> GAMGSMSKSLKKLVEESREKNQPEVDMSDRGISNMLDVNGLFTLSHITQLVLSHNKLTMVPPNIAELKNLEVLNFFNNQIEELPTQISSLQKLKHLNLGMNRLNTLPRGFGSLPALEVLDLTYNNLSENSLPGNFFYLTTLRALYLSDNDFEILPPDIGKLTKLQIL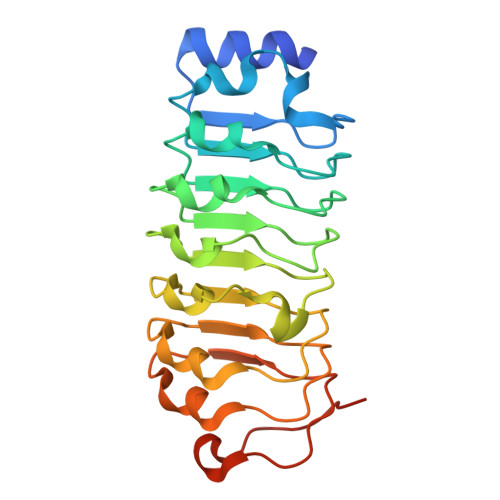SLRDNDLISLPKEIGELTQLKELHIQGNRLTVLPPELGNLDLTGQKQVFKAEN>[2x]MRSRRVDVMDVMNRLILAMDLMNRDDALRVTGEVREYIDTVKIGYPLVLSEGMDIIAEFRKR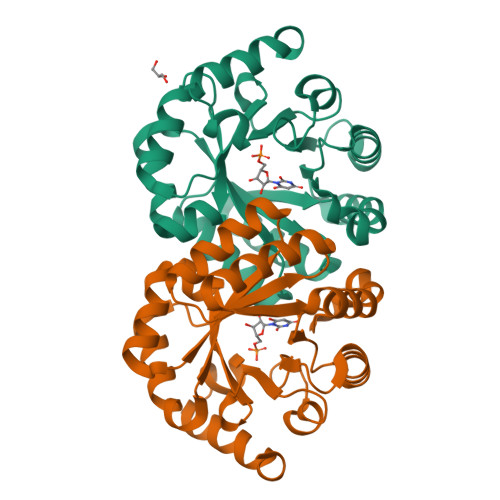FGCRIIADFKVADIPETNEKICRATFKAGADAIIVHGFPGADSVRACLNVAEEMGREVFLLTEMSHPGAEMFIQGAADEIARMGVDLGVKNYVGPSTRPERLSRLREIIGQDSFLISPGAGAQGGDPGETLRFADAIIVGRSIFLADNPAAAAAGIIESIKDLLNP> MAVHLTRIYTRTGDDGTTGLSDMSRVAKTDARLVAYADCDEANAAIGAALALGHPDTQITDVLRQIQNDLFDAGADLSTPIVENPKHPPLRIAQSYIDRLEGWCDAYNAGLPALKSFVLPGGSPLSALLHVAR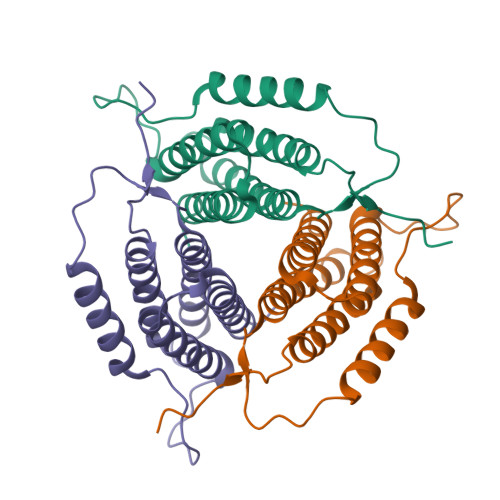TVVRRAERSAWAAVDAHPEGVSVLPAKYLNRLSDLLFILSRVANPDGDVLWRPGGDRTAS> XATTPL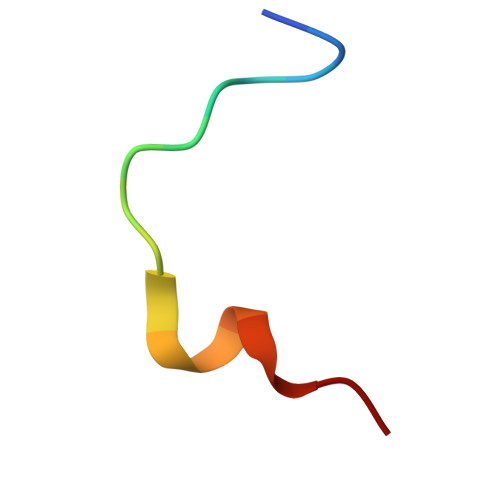CGPSRASILSG> AEDDPYLGRPEQMFHLDPSLTHTIFNPEVFQ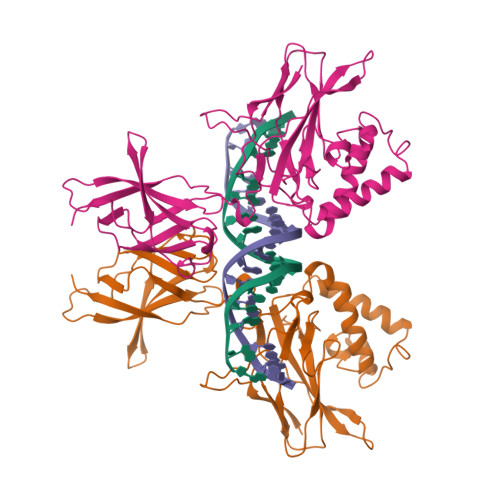PQMALPTADGPYLQILEQPKQRGFRFRYVAEGPSHGGLPGASSEKNKKSYPQVKICNYVGPAKVIVQLVTNGKNIHLHAHSLVGKHCEDGICTVTAGPKDMVVGFANLGILHVTKKKVFETLEARMTEACIRGYNPGLLVHPDLAYLQAEGGGDRQLGDREKELIRQAALQQTKEMDLSVVRLMFTAFLPDSTGSFTRRLEPVVSDAIYDSKAPNASNLKIVRMDRTAGCVTGGEEIYLLCDKVQKDDIQIRFYEEEENGGVWEGFGDFSPTDVHRQFAIVFKTPKYKDINITKPASVFVQLRRKSDLETSEPKPFLYYPEIKDKEEVQRKRQK> SKGLEDSSTISFITWNIDGLDGCNLPERARGVCSCLALYSPDVVFLQEVIPPYCAYLKKRAASY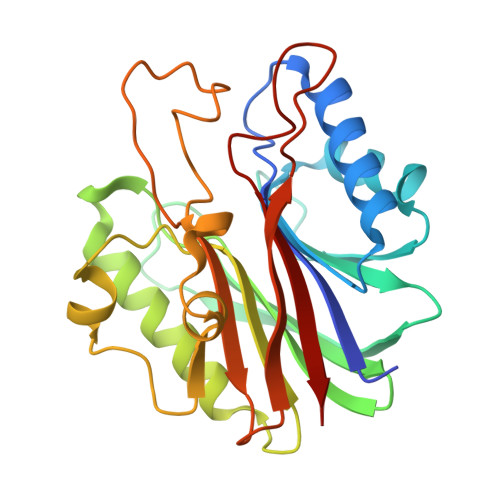TIITGNEEGYFTAILLKKGRVKFKSQEIIPFPNTKMMRNLLCVNVSLGGNEFCLMTSHLESTREHSAERIRQLKTVLGKMQEAPDSTTVIFAGDTNLRDQEVIKCGGLPDNVFDAWEFLGKPKHCQYTWDTKANNNLRIPAAYKHRFDRIFFRAEEGHLIPQSLDLVGLEKLDCGRFPSDHWGLLCTLNVVL>HHHHHHASENLYFQGAMASEKHFKYVILGGGVAAGYAAREFAKQGVKPGELAIISKEAVAPYERPALSKGYLFPQNAARLPGFHVCVGSGGERLLPEWYSEKGIELILSTEIVKADLASKTLTSAVGATFTYEILIIATGSSVIKLSDFGTQGADSNNILYLREVDDADKLVAAIQAKKGGKAVIVGGGYIGLELSAALKINDFDVTMVFPAPWCMPRLFTADIAAFYESYYTNKGVKIVKGTVAVGFDADANGDVTAVNLKNGSVLEADIVVVG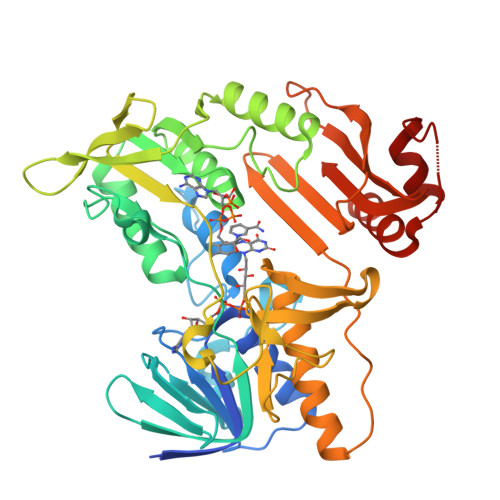VGGRPLTTLFKGQVAEEKGGIKTDAFFETSVPGVYAVGDVATFPMKMYNELRRVEHVDHARKSAEQAVKAIKGKESGESVVEYDYLPYFYSRSFDLGWQFYGDNVGDTILFGDSDPTSAKPKFGSYWIKDGKVLGAFLEGGSPDENKAIAKVAKTQPPVANIEELKKEGLQFASKI[2x]>MHHHHHHLKNGMRPIHPGEILREEFQKEMGFSAAALARALGVATPTVNNILRERGGVSADMALRLSICLDTTPEFWLNLQTAFDLRTAEQQHGDEIIGSVQRLVA[4x]

GraTA (Growth rate affecting Toxin–Antitoxin) is a type II TA module recently discovered in Pseudomonas putida. By sequence similarity, GraTA is most closely related to the higBA TA family. Here we show that GraA does not contain unstructured regions and forms a globular dimer while the toxin GraT contains an N-terminal intrinsically disordered region that is key for transcriptional regulation of the graTA operon as well as for the RNase activity of GraT. GraA binds tightly to the graTA operator and GraT prevents this interaction through steric interference from its N-terminal disordered region.

We determined the crystal structure of GraA2 in complex with the full 33 bp operator at 3.8 Å resolution. Surprisingly, in the crystal two non-interacting GraA dimers bind at opposite sides of the double helix. The total buried surface area between the two GraA dimers and the DNA is 2234 Å2. Each GraA2 has one of its HTH motifs interacting with the central TAACGTTA palindrome. This “central binding” HTH motif binds with its interaction helix α3 to a TAAC half palindrome. No hydrogen bonds between the protein and the DNA bases are observed. The other HTH motifs of each GraA2 act as the “support” subunits and interact with two distal half sites with sequences TAAG and TAAC, respectively. In these distal half sites the interaction is again directed towards the DNA phosphate backbone, and no base-specific contacts are made between protein and DNA. Binding does not affect the conformation of the GraA monomer nor the relative position or orientation of the monomers in the dimer.>[2x]MHSMKLLVTGGMGFIGSNFIRYILEKHPDWEVINIDKLGYGSNPANLKDLEDDPRYTFVKGDVADYELVKELVRKVDGVVHLAAESHVDRSISSPEIFLHSNVIGTYTLLESIRRENPEVRFVHVSTDEVYGDILKGSFTENDRLMPSSPYSATKAASDMLVLGWTRTYNLNASITRCTNNYGPYQFPEKLIPKTIIR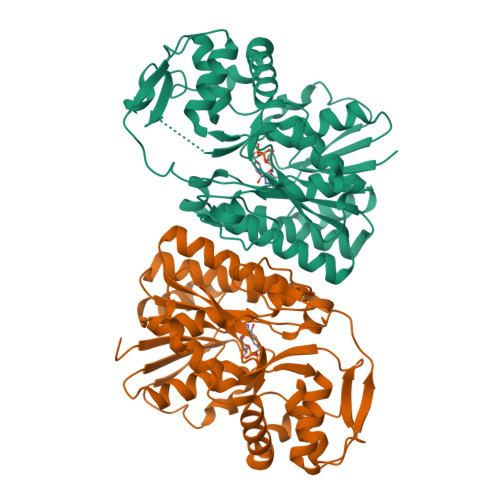ASLGLKIPIYGTGKNVRDWLYVEDHVRAIELVLLKGESREIYNISAGEEKTNLEVVKIILRLMGKGEELIELVEDRPGHDLRYSLDSWKITRDLKWRPKYTFDEGIKKTIDWYLKNEWWWKPLVDERILHPTPWKLKW> MNSAE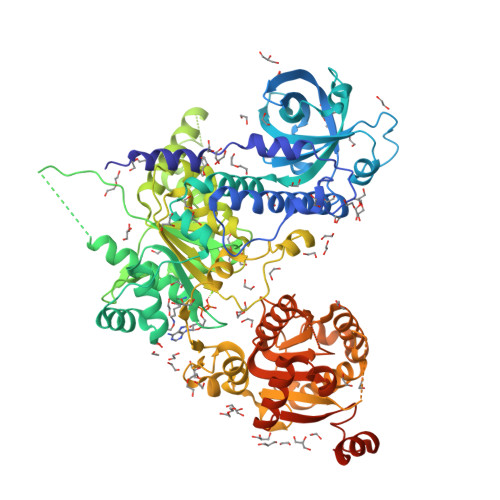LAKQELEHMRKRLNVDMNPLYEIILQWDYTRNSEYPDDEPIGNYSDVKDFFNSPADYQKVMKPLLLLESWQGLCSSRDREDYKPFSIIVGNRTAVSDFYDVYASVAKQVIQDCGISESDLIVMAYLPDFRPDKRLSSDDFKKAQHTCLAKVRTLKNTKGGNVDVTLRIHRNHSFSKFLTLRSEIYCVKVMQMTTIEREYSTLEGLEYYDLVGQILQAKPSPPVNVDAAEIETVKKSYKLNTSQAEAIVNSVSKEGFSLIQGPPGTGKTKTILGIIGYFLSTKNASSSNVIKVPLEKNSSNTEQLLKKQKILICAPSNAAVDEICLRLKSGVYDKQGHQFKPQLVRVGRSDVVNVAIKDLTLEELVDKRIGERNYGSGSKNSVNYRNRDLDRRNAQAHILAVSDIICSTLSGSAHDVLATMGIKFDTVIIDEACQCTELSSIIPLRYGGKRCIMVGDPNQLPPTVLSGAASNFKYNQSLFVRMEKNSSPYLLDVQYRMHPSISKFPSSEFYQGRLKDGPGMDILNKRPWHQLEPLAPYKFFDIISGRQEQNAKTMSYTNMEEIRVAIELVDYLFRKFDNKIDFTGKIGIISPYREQMQKMRKEFARYFGGMINKSIDFNTIDGFQGQEKEIILISCVRADDTKSSVGFLKDFRRMNVALTRAKTSIWVLGHQRSLAKSKLWRDLIEDAKDRSCLAYACSGFLDPRNNRAQSILRKFNVPVPSEQEDDYKLPMEYITQGPDEVKSN> GPGSYPSSNTLVE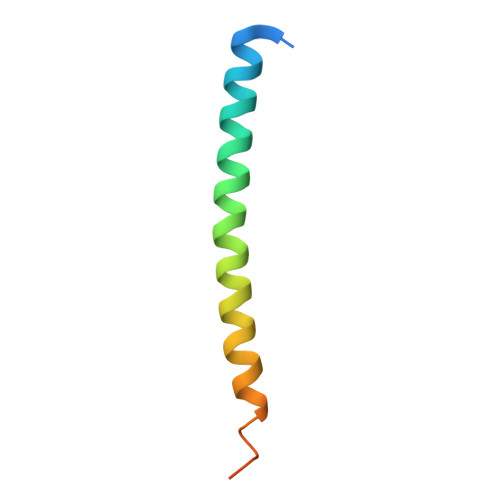MTLGMKKLKEEMEGVVKELAENNHILERFGSLTMDGGLRNVDCL4-(2-chloranylethanoyl)-~{N}-[(4-methoxyphenyl)methyl]-1-(4-methoxyphenyl)sulfonyl-piperazine-2-carboxamide 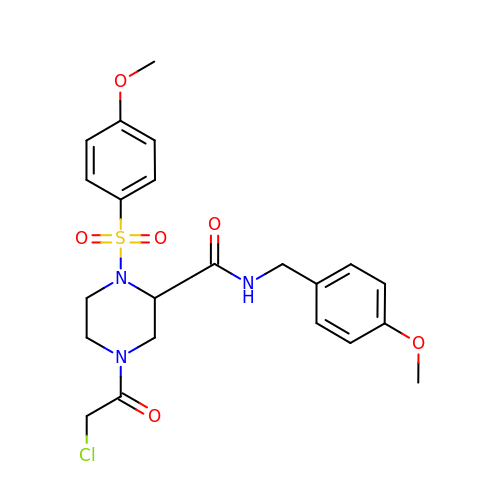| C22 H26 Cl N3 O6 S | SXQZEMXQTRNLRZ-HXUWFJFHSA-N> SAAPKAGTATGQIVAVIGAVVDVQFDEGLPPILNALEVQGRESRLVLEVAQHLGESTVRTIAMDGTEGLVRGQKVLDSGAPIKIPVGPETLGRIMNVIGEPIDERGPIKTKQFAPI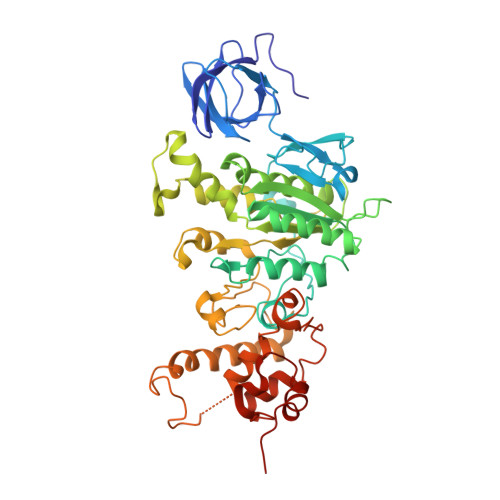HAEAPEFIEMSVEQEILVTGIKVVDLLAPYAKGGKIGLFGGAGVGKTVLIMELINNVAKAHGGYSVFAGVGERTREGNDLYHEMIESGVINLKDATSKVALVYGQMNEPPGARARVALTGLTVAEYFRDQEGQDVLLFIDNIFRFTQAGSEVSALLGRIPSAVGYQPTLATDMGTMQERITTTKKGSITSVQAIYVPADDLTDPAPATTFAHLDATTVLSRAIAELGIYPAVDPLDSTSRIMDPNIVGSEHYDVARGVQKILQDYKSLQDIIAILGMDELSEEDKLTVSRARKIQRFLSQPFQVAEVFTGHMGKLVPLKETIKGFQQILAGDYDHLPEQAFYMVGPIEEAVAKADKLAEEHGS tert-butyl 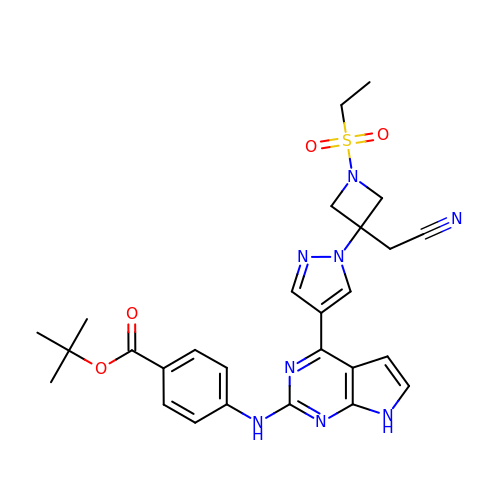4-[(4-{1-[3-(cyanomethyl)-1-(ethylsulfonyl)azetidin-3-yl]-1H-pyrazol-4-yl}-7H-pyrrolo[2,3-d]pyrimidin-2-yl)amino]benzoate | C27 H30 N8 O4 S | XPNMPGAYHLKXMY-UHFFFAOYSA-N> FTRLCREKTQEIYPIKEANGRTRKALIICNTEFKHLSLRYGANFDIIGMKGLLEDLGYDVVVKEELTAEGMESEMKDFAALSEHQTSDSTFLVLMSHGTLHGICGTMHSEKTPDVLQYDTI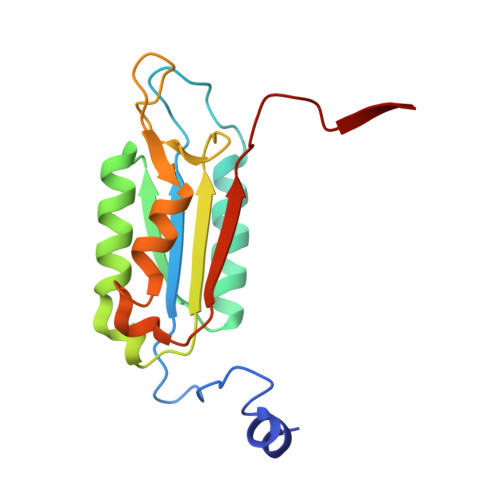YQIFNNCHCPGLRDKPKVIIVQAARGGNSGEMWI>[2x]GSMILYDLQQNLSSSH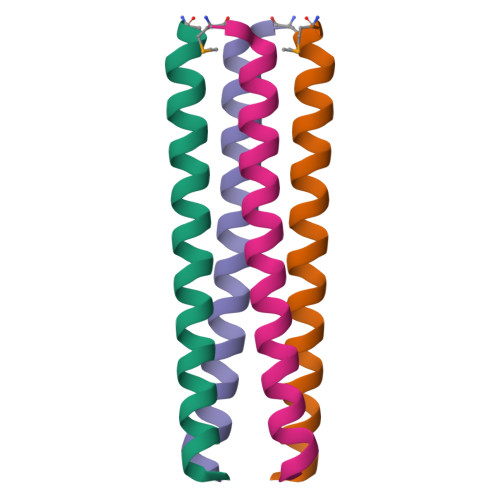RALEKQIDTLAGKLDALTELLSTALG{5-[(DIFORMYLAMINO)METHYL]-1-BENZOTHIEN-2-YL}BORONIC ACID | C11 H10 B N O4 S | 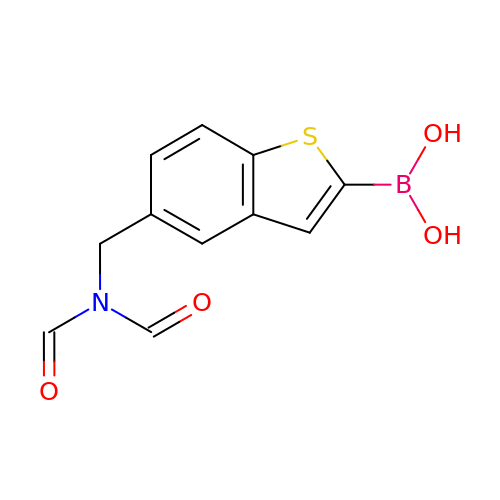GVTZPLCQJFQOTQ-UHFFFAOYSA-N>[2x]MAHHHHHHMAEFSIIDQYFNRQSHPDVALGIGDDSALITPPPNQQLVICADTLVAGRHFPLETSPHAIGWKSVAVNLSDIAAMGAKPHSILLAISLPQVDHEWLEGFSQGIYDCCNQFGVALIGGDTTQGPHLTITVTAMGWIETGKAVLRSGAKVGDYVCVSGQIGDAAYGLQHLGHSLQQRLDYPTPRCKLGEELKGLASSMIDVSDGLAQDLGHILKASKVGARLILEKLPVDPVLQQIEEQQRWQYALAGGDDYELCFTITPQNYEKLLQKQLDVKITMIGQIVEQTKLTFEHLGSDYPLQIHGYQHFAQQRW

Thiamine pyrophosphate (TPP) is the biologically active form of vitamin B1 (thiamine) and is essential for all living organisms. The same study also identified genes essential for growth on nutrient agar using high-density transposon mutagenesis, and found thiamine monophosphate kinase (ThiL) to be essential. In this study, we present high-resolution crystal structures of ThiL from the pathogen Acinetobacter baumannii (AbThiL) bound to substrate Thiamine monophosphate (TMP) and substrate analog adenylyl-imidodiphosphate (AMPPNP), and bound to its products TPP and adenosine diphosphate (ADP). The AbThiL structures assume the same two domain fold as MfThiL and AaThiLwith an N-terminal A domain and a C-terminal B domain.

Crystals grown in the presence of 5 mM AMPPNP/TMP/MgCl2 had many growth defects. Hence, co-crystals of AbThiL with 5 mM AMPPNP/MgCl2 from an optimization screen based on MCSG1 G4 (19% w/v PEG 3350, 200 mM K/Na-tartrate, 100 mM HEPES/NaOH pH 7.5) were soaked overnight with 5 mM AMPPNP/TMP/MgCl2. Crystals were harvested in two steps with reservoir with 20% v/v EG, 5 mM AMPPNP/TMP/MgCl2 added as the cryo protectant. The AMPPNP/TMP data set was collected at the APS LS-CAT beamline 21-ID-F equipped with a C(111) monochromator, and a Rayonix MX-225 detector. For the AMPPNP/TMP structure an anomalous signal could be detected for the potassium site, despite the weaker anomalous signal at shorter wavelength. For this structure, potassium was part of the crystallization condition. One metal that is in the center of the reaction is consistently magnesium: In the substrate complex a magnesium ion complexes both the scissile phosphoester bond in ATP, γ-phosphate and β-phosphate, and also the uncleaved β-phosphate and α-phosphate. Similarly, in the AbThiL substrate complex (AMPPNP/TMP), the α-phosphate group of TMP is already positioned for an in-line attack on the non-hydrolyzable γ-phosphate group of AMPPNP. In addition, we observed that the product complex (ADP/TPP) has a very similar conformation as the substrate complex. A superposition of the product complex and the substrate complex of AbThiL highlighs that the α-phosphate of TMP/TPP, and the α-phosphate and the β-phosphate groups of AMPPNP/ADP virtually do not move.>[2x]MDIAKRCESNPLLSPKDLKAGINDMEITCLLNPGVFKFKGKTWLLLRVAERPVQQEGIISFPIYDEQGQIKVMSFAENDPDLDASDPRVIGYKGKNYLTTMSYLRLVSSEDGIHFHDEPGYPPIFGKGELEAFGIEDCRVASTKDGFYLTFTEVSSVAVGVGMMHTNDWKTFEHY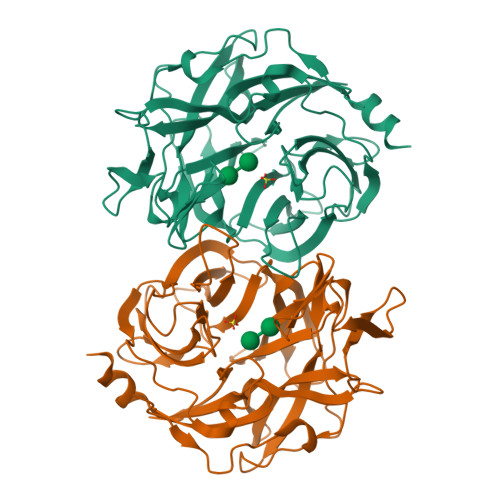GMILPPHNKDCALFEEKINDKYYTFHRPSSPELGGNYIWLAESPDLRHWGNHKCVATTRDGFWDCARVGAGAAPIKTEAGWLEIYHGADFNHRYCLGALLLDLNDPSKVLARSKEPIMEPIASYEQTGFFGNVIFTNGQLVDGDTITIYYGASDEVICKAELSVKEILNILNVGILEHHHHHH>MGSVADTVARVLRGCLENMPEADCIPKEQLSTSFQWVTKWVDYSNKYGFGYQLSDHTVGVLFNNGAHMSLLPDKKTVHYYAELGQCSVFPATDAPEQFISQVTVLKYFSHYMEENLMDGGDLPSVTDIRRPRLYLLQWLKSDKALMMLFNDGTFQVNFYHDHTKIIICSQNEEYLLTYINEDRISTTFRLTTLL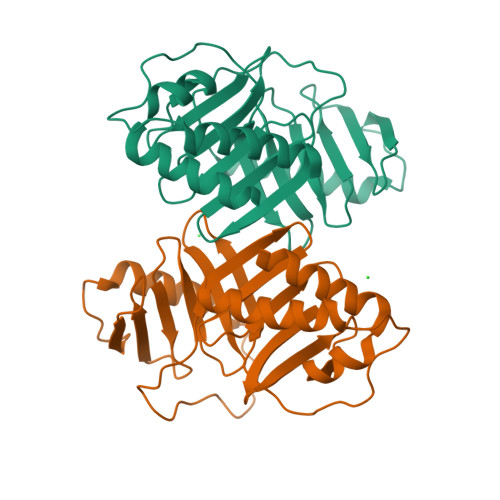MSGCSSELKNRMEYALNMLLQRCN[2x]>GSPSTRDYEIQRERIELGRCIGEGQFGDVHQGIYMSPENPALAVAIKTCKNCTSDSVREKFLQEALTMRQFDHPHIVKLIGVITENPVWIIMELCTLGELRSFLQVRKYSLDLASLILYAYQLSTALAYLES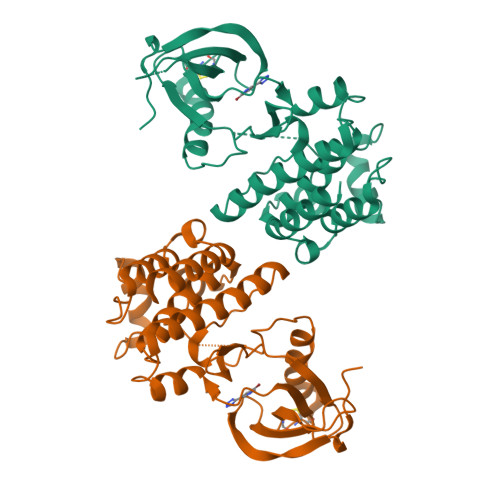KRFVHRDIAARNVLVSSNDCVKLGDFGLSRYMEDSTYYKASKGKLPIKWMAPESINFRRFTSASDVWMFGVCMWEILMHGVKPFQGVKNNDVIGRIENGERLPMPPNCPPTLYSLMTKCWAYDPSRRPRFTELKAQLSTILEEEKAQ[2x]> MADNYVIWFENLRMTDVERVGGKNASLGEMISQLTEKGVRVPGGFATTAEAY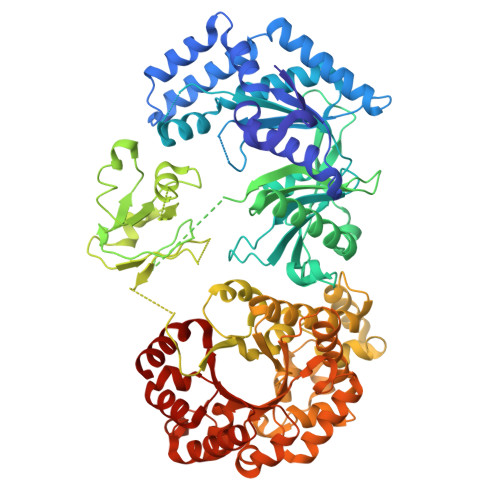RAFLAHNGLSERISAALAKLDVEDVAELARVGKEIRQWILDTPFPEQLDAEIEAAWNKMVADAGGADISVAVRSSATAEDLPDASFAGQQETFLNINGLDNVKEAMHHVFASLYNDRAISYRVHKGFEHDIVALSAGVQRMVRSDSGASGVMFTLDTESGYDQVVFVTSSYGLGENVVQGAVNPDEFYVFKPTLKAGKPAILRKTMGSKHIKMIFTDKAEAGKSVTNVDVPEEDRNRFSITDEEITELAHYALTIEKHYGRPMDIEWGRDGLDGKLYILQARPETVKSQEEGNRNLRRFAINGDKTVLCEGRAIGQKVGQGKVRLIKDASEMDSVEAGDVLVTDMTDPDWEPVMKRASAIVTNRGGRTCHAAIIARELGIPAVVGCGNATELLKNGQEVTVSCAEGDTGFIYAGLLDVQITDVALDNMPKAPVKVMMNVGNPELAFSFANLPSEGIGLARMEFIINRQIGIHPKALLEFDKQDDELKAEITRRIAGYASPVDFYVDKIAEGVATLAASVYPRKTIVRMSDFKSNEYANLVGGNVYEPHEENPMLGFRGAARYVADNFKDCFALECKALKRVRDEMGLTNVEIMIPFVRTLGEAEAVVKALKENGLERGKNGLRLIMMCELPSNAVLAEQFLQYFDGFSIGSNDMTQLTLGLDRDSGLVSESFDERNPAVKVMLHLAISACRKQNKYVGICGQGPSDHPDFAKWLVEEGIESVSLNPDTVIETWLYLANELNK> QISQAIKYLQNNIKGFIIRQRVNDEMKVNCATL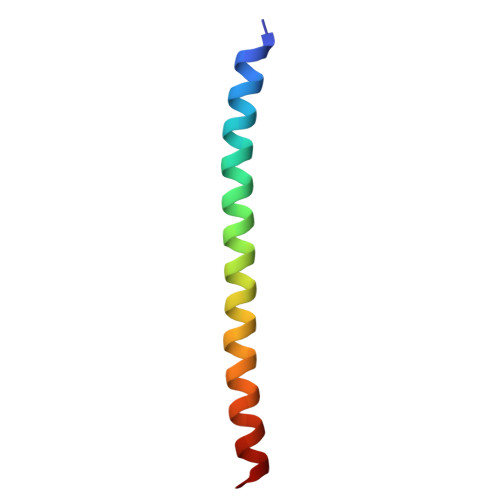LQAAYRGHSIRANVF PYRAZOLE | 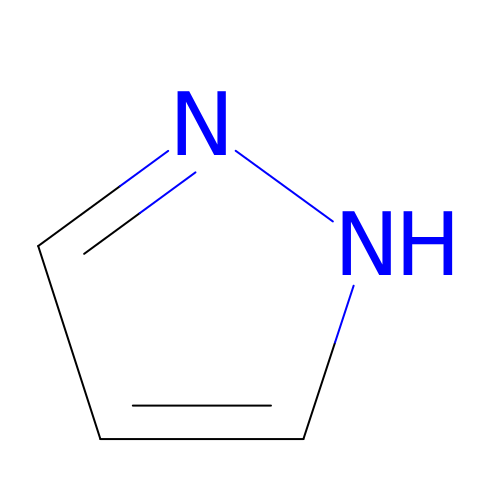C3 H4 N2 | WTKZEGDFNFYCGP-UHFFFAOYSA-N>MGSSHHHHHHSQDPGINRKAINFDLSTKSLEKYFKDTREPYSLIKKFMLENGFEHRQYSGYTSKEPINERRVIRIINKLTKKFTWLGECVKEFDITEIGEQYSLKETIQDLCAKDFHQKLKEFTEKTPKNQKLKDLER[2x];>[2x]MASMTGGLEHPQFEKLEQKLISE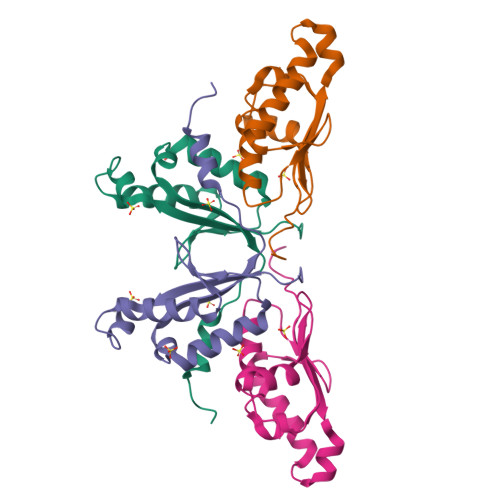EDLEDLAYPLLGTRIVLDEEKILKEGKYNLEDMYKMIDEYAKESGMIKINKETYHCKGDKYDLGCMTLFIYKYLIDSEWFTKNAKEWIWISEKEGNSDLISASKAEGEGIWE>[2x]MVRPSQSMYDRHLTIFSPDGNLYQIEYAIKAVKNTNITSVGVKGENCAVIISQKKMATQYISQDKLLDYNNITNIYNIT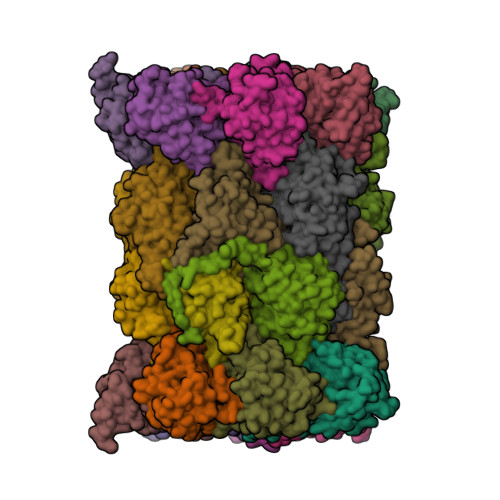DEIGCSMVGMPGDCLSMVYKARSEASEFLYSNGYNVNAETLCRNICDKIQVYTQHAYMRLHACSGMIIGIDENNKPELFKFDPSGFCAGYRACVIGNKEQESISVLERLLEKRKKKIQQETIDEDIRNTTILAIEALQTILAFDLKASEIEVAIVSTKNRNFTQISEKEIDNYLTYIAERD;>MADGEYSFSLTTFSPTGKLVQIEYALNRVSSSSPALGIRAKNGVIIATEKKSPNELIEENSIFKIQQISEHIGIVYAGMPGDFRVLLKRARKEAIRYSLQYGSEILVKELVKIIASIVQEFTQTGGVRPFGLSLLICGVDVYGYHLYQIDPSGCYFNWMATCVGKDYQNNMSFLEKRYNKDIEIEDAIHTAILTLKESYEGVLNEKNIEIGVAYDNKPFKILTQNEIKDYLIEIE[2x];>[2x]MARRYDSRTTTFSPEGRLYQVEYALEAINNASITIGLITKDGVILGADKVFISKLIDKANNYEKIYKIDKHIFCGVAGLNADANILINQSRLYAQRYLYNYNEVQPVSQLVVQICDIKQSYTQYGGLRPYGVSFLIGGYDTKDGYQLYHTDPSGNYSGWFATAIGTNNLTASSVLKQEWKNDMTLEEGLLLALKTLAKSTDTEIPKSEKIELAYLTNKDGEVYQKYLTEKEIEELIKLYTQKYIKE;>MSYDRAITVFSPDGHLLQVEHALEAVKKGGCAVAIKSSNFAVLAVEKKNIPKLQNPKTTEKLIKLDEHNCLAFAGLNADARVLVNKTRLECQRYYLNMDEPAPVDYIAKYVAKVQQKFTHRGGVRPFGIATLIAGFKNNKEICIYQTEPSGIYAAWKAQAIGKNAKIVQEFLEKNYQENMEQKDCIFLALKAIFEVVELSSKNVEVALLTEKDLTFIEEQEINSMVELIDQERTKNNEQNE[2x];>[2x]MFSTRSEYDRGVNTFSPEGRLFQVEYALGAIKLGSTAVGICVNDGVILASERRISSTLIEKDSVEKLLSIDDHIGCAMSGLMADARTLIDYARVECNHYKFIYNENINIKSCVELISELALDFSNLSDSKRKKIMSRPFGVALLIGGVDKNGPCLWYTEPSGTNTRFSAASIGSAQEGAELLLQENYKKDMTFEQAEILALTVLRQVMEDKLSTSNVEICAIKKSDQTFYKYNTDDISRIIDVLPSPVYPTIDMTA;>[2x]MYRNLYDTDNIIYSPEGRLYQVEYASEAIKQGTCAVAIKSKDYVVVSGLKKCISKLSFPQEKIFKIDDYIGISMSGITSDAKVLTKFMQNECLSHKFLYNENINIESLVRSVADKYQKNTQKSSKRAFGVGLMIAAYHNEPCIFETRPNGSYFEYDALSFGARSHASKTYLEKNLHLFEECSLEELILHCLKALKCSLSSESELTISNTALAVVGKNHPWQEISSLQLEEYLSKVKMDAEQEQVEENVQNEANE;>[2x]MAGLSAGYDLSVSTFSPDGRLYQVEYIYKSINNNNTALCLECKDGIICCCINSNMDKNKMIKKNSYNRIYHVNNNIIITYSGFDGDARNIIDRARSEANTYYYNFHTNIPLHILVNRISLYIHAYTLYWHMRPFAASIIISSFNEKDKGDIYCIEPNGACYKYSGIVIGKNKEMFKTEIEKKDYKDINVRDAIEDIYKFILTSDDHMNKNNLQNLVNFSWICKESSYEFQNIHEEILTPALNKAVEYIEKLN;>[2x]TTIIGIIYDNGVMLACDSRTSSGTFISNKCSRKINRINENLYVCRSGASAHSQKIIEIIKHYCVSMKNENRKKGRFHEGETIYDETTYDEEIDIDSINYLDYNNNNDNNLVTKNKYFYEDKFNDYNPLVENVAHITKKIIYTNNNFLSCALIFGGYDKIKKQQLYAVNLNGSIIEKHDFAVSGSGSIYIQSYLQDKYKKFMTKKECFNLILNCVKYAMHNDNSSGGLIRIVNITKSFVEEFTVVNTQMNFQY;>TTICGLVCQNAVILGADTRATEGPIVADKNCSKLHYISKNIWCAGAGVAGDLEHTTLWLQHNVELHRLNTNTQPRVSMCVSRLTQELFKYQGYKVCAIVLGGVDVNGPQLYGIHPHGSSCLLPFTALGSGSLNAMAVLEAKYRDNMTIEEGKNLVCEAICAGIFNDLGSGGNVDICVITKDSYQHIRPYKEPNMRLYHLPHPTIYPKGTTPILSEKIEYIKKFISVEDA[2x];>MGSIYNYNGGCVLGMSGSNCVAIACDLRLGANTFTTVSTKFSKIFKMNNNVYVGLSGLATDIQTLYEILRYRVNLYEVRQDAEMDVECFANMLSSILYSNRFSPYFVNPIVVGFKLKHYVDEEGEKKVNYEPYLTAYDLIGAKCETRDFVVNGVTSEQLFGMCESLYVKDQDENGLFETISQCLLSALDRDCISGWGAEVLVLTPEKIIKKKLKARMD[2x];>[2x]MDTLIGLRGNNFVVLAADTYSINSIIKLKNDDNTKFYDIHGNKCLLLGGSIGDRLQFGEFIRKNVHLYQYQNNTDMFVKSFAFFTRKNLAYYLRRNPFEVNCLIAGYDKKDGYQLYWCDYLSNMDSVNKGAHGYGAYLVSAILDKYYHENLTVDEALDIFKLCFEELKKRFLLTQINYELRIMYDNKVETQYVTV;>[2x]TTTLAFKFKDGIIVAVDSRASMGSFISSQNVEKIIEINKNILGTMAGGAADCLYWEKYLGKIIKIYELRNNEKISVRAASTILSNILYQYKGYGLCCGIILSGYDHTGFNMFYVDDSGKKVEGNLFSCGSGSTYAYSILDSAYDYNLNLDQAVELARNAIYHATFRDGGSGGKVRVFHIHKNGYDKIIEGEDVFDLHYHYTNPEQKDQYVM;>[2x]MDLILYNDNLTEKKTEKENVIEHGRGFKRWYPYIDNGGTVIGLTGKDYVILAADTRLSLSYSIYTRFCPKISKLTDKCIIGSSGMQSDIKTLHSLLQKKIQLFVLEHSHYPDIHVIDRLLCVILYSRRFFPYYAFNILAGVDENNKGVLYNYDSVGSYCEATHSCVGSGSQLILPILDNRVEQKNQLIKNTNFNLGDDINFVKDAITSATERDIYTGDKTLIYVIDKMGINVNTLDLKQD;>MTLGPVVTGTSVIAIKYKHGIMIAADRKASYGSYAKFQNVERIFKINNKTVMGFSGELADAQYLHELLTRKNINNLSEKKRKEDMYTPQHYHSYVSRVFYVRKNRIDPLFNNIIIAGINSQKYDNNDDNVLLYTNKNNDDEQNEYKNNEEYKEIHKDDLYIGFVDMHGTNFCDDYITTGYARYFALTLLRDHYKDNMTEEEARILINECLRILYFRDATSSNFIQIVKVTSKGVEYEEPYILPCVLNSADYVYPSTLLPPAGCMW[2x]2-(1H-imidazol-1-yl)ethyl dimethylcarbamate | C8 H13 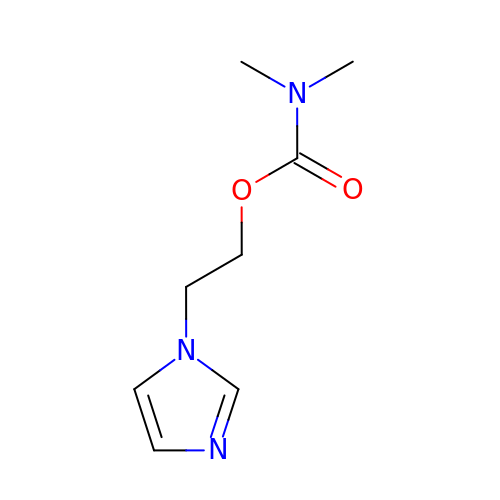N3 O2 | WSDMJRGHLMKKID-UHFFFAOYSA-N> RSMSRPVQEMIPLKFFAVDEVSCQINQEGAPKDVVEKVLFVLNNVTLANLNNKVDELKKSLTPNYFSWFSTYLVTQRAKTEPNYHDLYSKVIVAMGSGLLHQFMVNVTLRQLFVLLSTKDEQAIDKKHLKNLASWLGCITLALNKPIKHKNIAFREMLIEAYKENRLEIVVPFVTKILQRASESKIFKPPNPWTVGILKLLIELNEKANWKLSLTFEVEVLLKSFNLTTKSLKPSNFINTPEVIETLSG;> RSMFLPPPNYLFVRDVWKSNLYSEFAVIRQLVSQYNHVSISTEFVGTLARPIGTFRSKVDYHYQTMRANVDFLNPIQLGLSLSDANGNKPDNGPSTWQFNFEFDPKKEIMSTESLELLRKSGINFEKHENLGIDVFEFSQLLMDSGLMMDDSVTWITYHAAYDLGFLINILMNDSMPNNKEDFEWWVHQ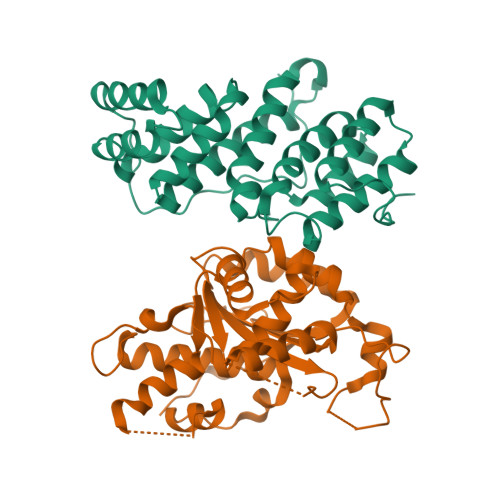YMPNFYDLNLVYKIIQEFKNPQLQQSSQQQQQQQYSLTTLADELGLPRFSIFTTTGGQSLLMLLSFCQLSKLSMHKFPNGTDFAKYQGVIYGIDGDQ> S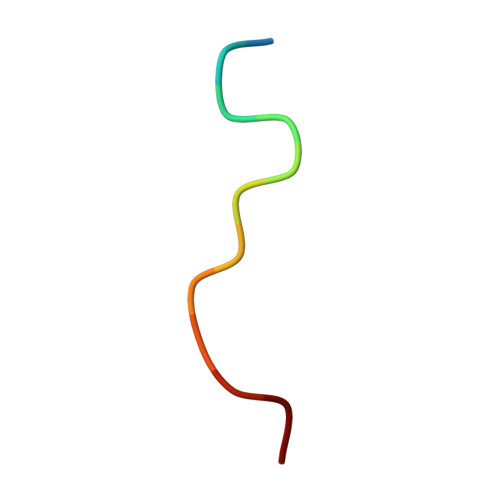NPNAGKVLLPTP>[2x]MGFKQDIATIRGDLRTYAQDIFLAFL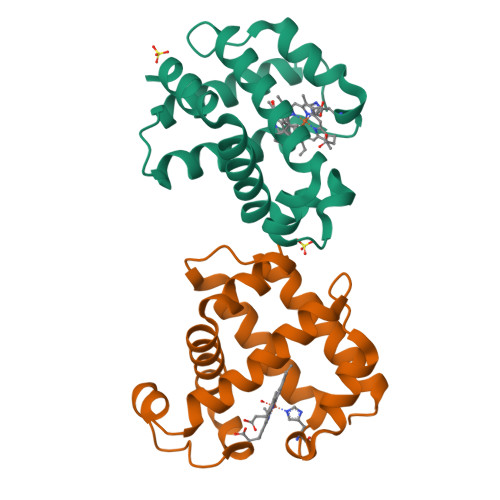NKYPDERRYFKNYVGKSDQELKSMAKFGDHTEKWFNLMMEVADRATDCVPLASDANTLVQMKQHSSLTTGNFEKLFVALVEYMRASGQSFDSQSWDRFGKNLVSALSSAGMK>GPQPPADEQPEPRTRRRAYLWCKEFLPGAWRGLREDEFHISVIRGGLSNMLFQCSLPDTTATLGDEPRKVLLRLYGAILQMRSCNKEGSEQAQKENEFQGAEAMVLESVMFAILAERSLGPKLYGIFPQGRLEQFIPSRRLDTEELSLPDISAEIAEKMATFHGMKMPFNKEPKWLFGTMEKYLKEVLRIKFTEESRIKKLHKLLSYNLPLELENLRSLLESTPSPVVFCHNDCQEGNILLLEGRENSEKQKLMLIDFEYSSYNYRGFDIGNHFCEWMYDYSYEKYPFFRANIRKYPTKKQQLHFISSYLPAFQNDFENLSTEEKSIIKEEMLLEVNRFALASHFLWGLWSIVQAKISSI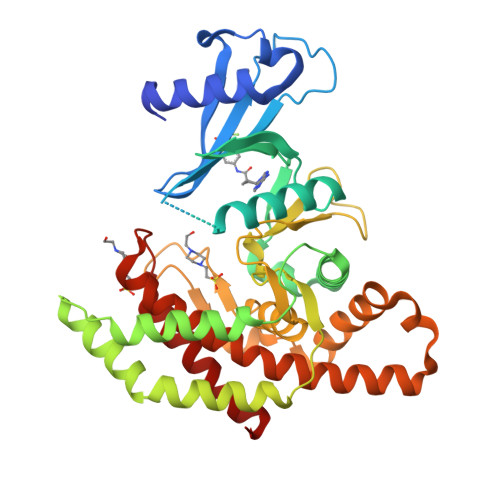EFGYMDYAQARFDAYFHQKRKLGV[2x]> GSAPLLLYANRRDLRLVDATNGKENATIVVGGLEDAAAVDFVFSHGLIYWSDVSEEAIKRTEFNKTESVQNVVVSGLLSPDGLACDWLGEKLYWTDSETNRIEVSNLDGSLRKVLFWQELDQPRAIALDPSSGFMYWTDWGEVPKIERAGMDGSSRFIIINSEIYWPNGLTLDYEEQKLYWADAKLNFIHKSNLDGTN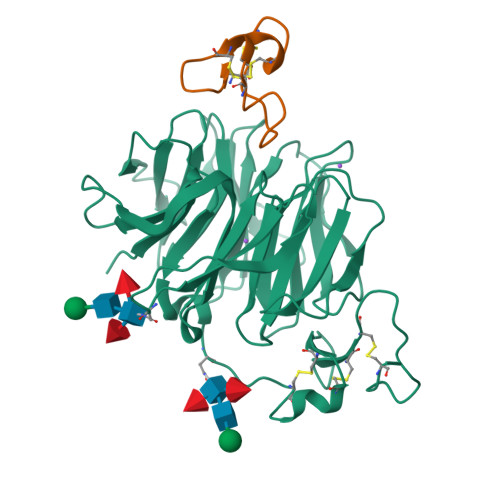RQAVVKGSLPHPFALTLFEDILYWTDWSTHSILACNKYTGEGLREIHSDIFSPMDIHAFSQQRQPNATNPCGIDNGGCSHLCLMSPVKPFYQCACPTGVKLLENGKTCKDGNSHHHHHH;> GCQSNHILKHNRCKQDSDCLAGCVCGPNGFCG> FSRPGLPVEYLQVPSPSMGRDIKVQFQSGGNN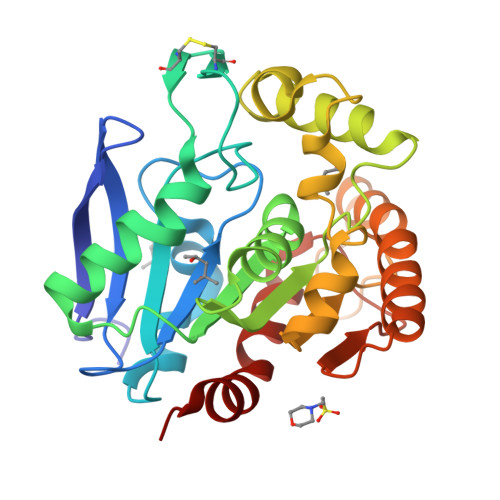SPAVYLLDGLRAQDDYNGWDINTPAFEWYYQSGLSIVMPVGGQSSFYSDWYSPACGKAGCQTYKWETFLTSELPQWLSANRAVKPTGSAAIGLSMAGSSAMILAAYHPQQFIYAGSLSALLDPSQGMGPSLIGLAMGDAGGYKAADMWGPSSDPAWERNDPTQQIPKLVANNTRLWVYCGNGTPNELGGANIPAEFLENFVRSSNLKFQDAYNAAGGHNAVFNFPPNGTHSWEYWGAQLNAMKGDLQSSLGAG The O-linked β-N-acetyl-d-glucosamine (O-GlcNAc) transferase (OGT) and the hydrolase O-GlcNAcase (OGA) together orchestrate protein O-GlcNAcylation, a dynamic co/posttranslational modification cycling on thousands of nucleocytoplasmic proteins. OGT catalyses the covalent attachment of the monosaccharide O-GlcNAc to serine or threonine. In addition to its glycosyltransferase activity, mammalian OGT is involved in the unusual proteolytic maturation of Host cell factor 1 (HCF1), a transcriptional cofactor implicated in cell cycle control, also identified as an ID gene. HCF1 is O-GlcNAc–modified and subsequently cleaved by OGT using the same active site for both enzymatic activities.

Here, we characterize an OGT missense mutation in the catalytic domain as observed in female twins with ID and developmental delay. In vitro biochemical analysis of recombinant N567K OGT missense variant protein revealed that this mutation abrogates OGT and HCF1 proteolytic processing activity. Inspection of the wild-type OGT structure reveals that Asn567 maps to a loop in the N-terminal lobe of the catalytic domain that is completely conserved through evolution from Caenorhabditis elegans to man. The Asn567 side chain borders the −2 subsite as part of the OGT acceptor substrate binding cleft. OGTN567K was then cocrystallized with a donor analog, UDP-5S-GlcNAc, and 2 OGT acceptor peptide substrates, P1 (KKVPVSRA) and P2 (KKVAVSRA), previously used for activity measurements. Only the condition containing P2, which contains an alanine at the −2 subsite, yielded crystals that diffracted to 2.3 Å and allowed structure solution by molecular replacement and refinement. The OGTN567K structure superposed onto that of OGTWT with an rmsd of 0.4 Å across 675 Cα atoms, suggesting the mutation does not induce large conformational changes in the catalytic domain. Surprisingly, this only covered the P2 backbone in the +2 through to −2 subsites, suggesting that the N567K mutation may induce increased flexibility at the N-terminal tail of the acceptor peptide. Close inspection of the OGTN567K acceptor substrate binding cleft revealed that the protrusion caused by the N567K mutation partially occupies the position of the −2 proline frequently observed in OGT acceptor peptides. Our structural analysis has uncovered that the N567K mutation changes the surface of the substrate binding pocket, thereby altering substrate binding ability of the N567K OGT.

> GPGSCPTHADSLNNLANIKREQGNIEEAVRLYRKALEVFPEFAAAHSNLASVLQQQGKLQEALMHYKEAIRISPTFADAYSNMGNTLKEMQDVQGALQCYTRAIQINPAFADAHSNLASIHKDSGNIPEAIASYRTALKLKPDFPDAYCNLAHCLQIVCDWTDYDERMKKLVSIVADQLEKNRLPSVHPHHSMLYPLSHGFRKAIAERHGNLCLDKINVLHKPPYEHPKDLKLSDGRLRVGYVSSDFGKHPTSHLMQSIPGMHNPDKFEVFCYALSPDDGTNFRVKVMAEANHFIDLSQIPCNGKAADRIHQDGIHILVNMNGYTKGARNELFALRPAPIQAMWLGYPGTSGALFMDYIITDQETSPAEVAEQYSEKLAYMPHTFFIGDHANMFPHLKKKAVIDFKSNGHIYDNRIVLNGIDLKAFLDSLPDVKIVKMKCPDGGDNADSSNTALNMPVIPMNTIAEAVIEMINRGQIQITINGFSISNGLATTQINNKAATGEEVPRTIIVTTRSQYGLPEDAIVYCNFNQLYKIDPSTLQMWANILKRVPNSVLWLLRFPAVGEPNIQQYAQNMGLPQNRIIFSPVAPKEEHVRRGQLADVCLDTPLCNGHTTGMDVLWAGTPMVTMPGETLASRVAASQLTCLGCLELIAKNRQEYEDIAVKLGTDLEYLKKVRGKVWKQRISSPLFNTKQYTMELERLYLQMWEHYAAGNKPDHMIKPVE;> KKVAVSRAA> MLEGKVKWFNSEKGFGFIEVEGQDDVFVHFSAIQGEGFKTLEEGQAVSFEIVEGNRGPQAANVTKE

BsCspB is a relatively small protein of 67 amino acids length that belongs to the cold shock protein family. Notably, BsCspB shows an overall thermodynamic stability of about ΔG° = 10 kJ mol−1 at T = 298 K and possesses fast unfolding, ku, and refolding, kf, rate constants of about ku = 12 s−1 and kf = 1070 s−1, respectively. In previous work, we have used auxotrophic E. coli strains to incorporate fluorinated phenylalanine (Phe) or tryptophan (Trp) amino acid residues into the Cold shock protein B from Bacillus subtilis (BsCspB). Our findings show that fluorine-labelling of proteins utilizing singly modified amino acids like Phe or Trp does not cause a detectable alteration of thermodynamic and structural properties of BsCspB.

Focusing on phenylalanine modified variants, 4-19F-Phe-BsCspB deviates most in ΔG° from wild type BsCspB by 1.5 kJ/mol. This property of 4-19F-Phe-BsCspB has been one rationale for the crystallization of this variant enabling to obtain atomically resolved information (see below). The fitting of Eq. to the data obtained for 4-19F-Phe-BsCspB using one-dimensional 19F NMR spectroscopy yield TM = 318.4 K and ΔH = 176 ± 6 kJ/mol confirming the thermodynamic analysis done by using 1H NMR spectroscopic data which has illuminated TM = 318.5 K. To investigate potential structural changes in 4-19F-Trp-BsCspB and 4-19F-Phe-BsCspB, we have elucidated their atomic structures using X-ray crystallography to 2.05 Å and 2.1 Å resolution, respectively. The samples crystallized in a closely related crystallographic lattice, containing one single molecular copy of modified BsCspB in the asymmetric unit and sharing a same space group symmetry. The global RMSD for all Cα atoms for the 4-19F-Trp-BsCspB and 4-19F-Phe-BsCspB structures calculated in this work is 0.23 Å, indicating that the fold trace of the two variants is virtually identical. Furthermore, wild type and 19F-derivative structures displayed identical conformational rotamers for the modified Trp and Phe residues, indicating that local structural distortions had also not taken place. Interestingly, these slight changes are independent of the number and sites of fluorine atoms which have been inserted into BsCspB: one fluorine atom used for 19F-Trp labelling (sequence position 8) or seven fluorine atoms used for 19F-Phe labelling (sequence positions 9, 15, 17, 27, 30, 38, and 49). To our knowledge, this represents the first three-dimensional structure determination of a fluorophenylalanine-labelled protein possessing more than a single fluorination site which has been reported so far. The analysis of both the unfolding and the refolding reaction of 4-19F-Phe-BsCspB leads to almost identical values for fN, namely fN = 0.191 and fN = 0.189, respectively. This result shows that 4-19F-Phe-BsCspB folds fully reversibly and that there is no apparent long-term folding rate constant additionally present which may explain the gap observed in the amplitude analysis of the kinetic data.> RVTLNIATNADSLGTWFLDAVSKFTGGSDYLVNIAVDDQDHTVEWLRGGRVLAAVTAHDKPVQGCRVTPLGVLRYHATASPDFMARHFADGVTPAALARAPGLTFNQKDRLQASWIRTALGEDVSYPTHWLPSTDGFVKASLAGMGWGLNPVQLVAEHLAAGRLVELMPGTPLDIPLYWQVNRLAAERLAGL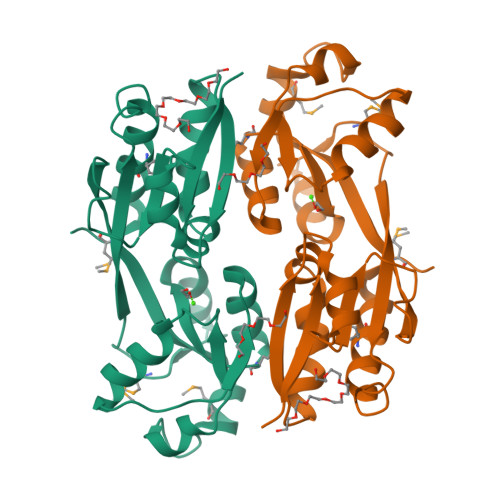TANMVGTARVVLMPVG>MTKTTDDNIIVGLDIGTATVSALVGEVLPDGQVNIIGAGSSPSRGMDKGGVNDLESVVKSVQRAVDQAELMAECQISSVFISLSGKHIASRIEKGMGTISEEEVSQDDMDRAIHTAKSIKIGDEQRILHVIPQEFTIDYQEGIKNPLGLSGVRMEVSVHLISCHNDMARNIIKAVERCGLKVEQLVFSGLASSNAVITEDERELGVCVVDIGAGTMDISIWTGGALRHTEVFSYAGNA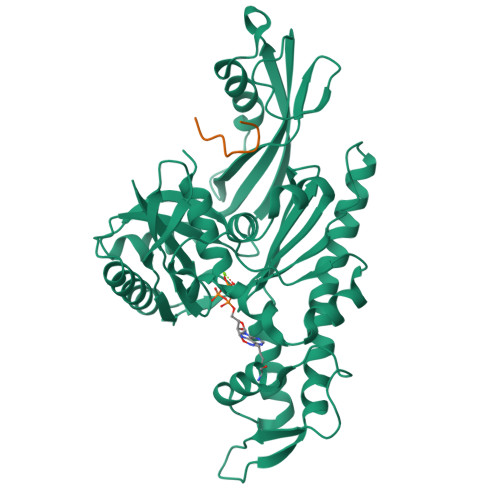VTSDIAFAFGTPLSDAEEIKVKYGCALSELVSKDDTVNVPSVGGRPSRSLQRQTLAEVIEPRYTELMGLVNQTIDNVQAKLRENGVKHHLAAGVVLTGGAAQIEGVVECAERVFRNQVRVGKPLEVSGLTDYVKEPYHSTAVGLLHYARDSQDNDDND[16x]>[2x]DRSRVFDILSNINIGWNLGNTLDATGGGNSVNAETSWGNPKTTQEIVDTVNDRGFNAIRIPVTFANHLGPAPEYTISADWLARVKEVVDYAVNDGMYIILDTHHETNYWLKTDPNNEAALCEELAAIWKQLAEAFKDYDEKLMFEGMNEPRMAGSAKEWSGGTPAERKLINA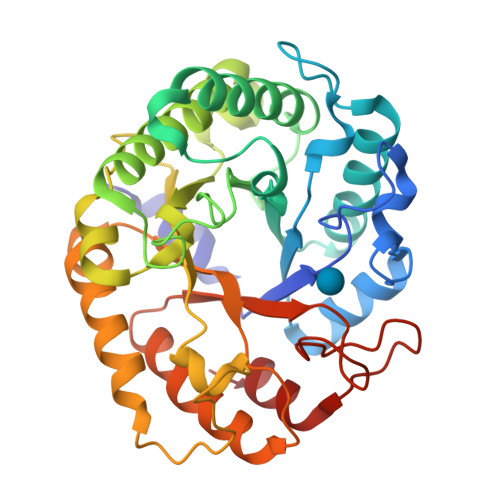MNKAFIDAVRATGGNNADRVLIICTYGHNSDEPTLKDLEIPSDPNIAVALHTYTPYFFTYVADGSYSVWNGSKKNDITWQYNNIKKYLIDKGIPVVITETGAQFKENTEDIVRWIGDYVGTLDQDGVKCFIWDNNIYHGNGEKFGLLNRSLLKWYNDDIVDAYVNHA> S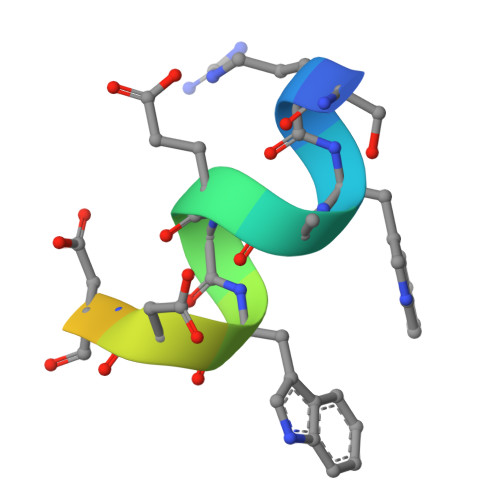RWAEVWDDNSKVSR>MKELNDLEKKYNAHIGVYALDTKSGKEVKFNSDKRFAYASTSKAINSAILLEQVPYNKLNKKVHINKDDIVAYSPILEKYVGKDITLKALIEASMTYSDNTANNKIIKEIGGIKKVKQRL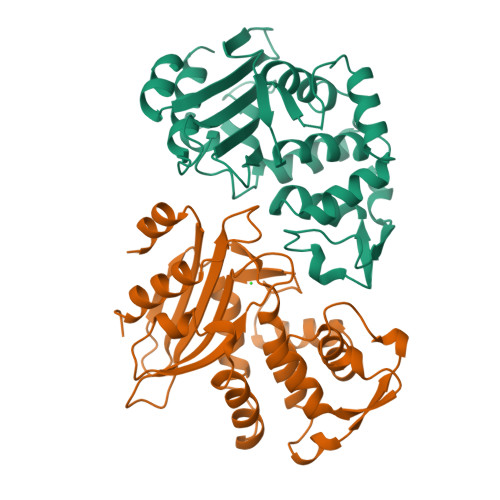KELGDKVTNPVRYEIELNYYSPKSKKDTSTPAAFGKTLNKLIANGKLSKENKKFLLDLMLNNKSGDTLIKDGVPKDYKVADKSGQAITYASRNDVAFVYPKGQSEPIVLVIFTNKDNKSDKPNDKLISETAKSVMKEF[2x]>IDTDAVVGDTIIDVSGKKMTIAEFYDSTPDVFMRRNDEARDWVKRVGGKTSLSVNTYSGEVERKNINYIMKHTVKKRMFKIKAGGKEVIVTADHSVMVKRDGKIIDVKPTEMKQTDRVVKWMLTGSHMIEFIEFEIEDLGVMEIDVYDIEVDGNHNFFGNDILVHASV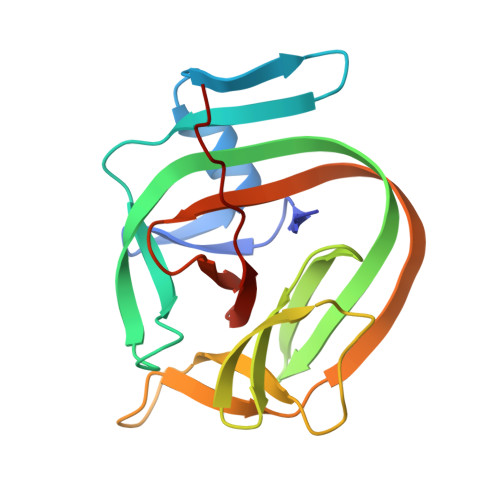YLNKL[2x]>GSHMEPPPKLVLDLERLAHVPQEKAGPLQRYAATIQSQRGDYNGKVLSIRQDDLRTLAVIYDQSPSVLTEQLISWGVLDADARRAVAHEEN[2x]

Here, we report that c-di-GMP can assemble into a tetramer that mediates the effective dimerization of a transcription factor, BldD, which controls the progression of multicellular differentiation in sporulating actinomycete bacteria. BldD is an 18 kDa DNA-binding protein consisting of two distinct domains connected by a flexible linker. BldD sits at the top of the regulatory cascade controlling development, serving to repress expression of sporulation genes during vegetative growth (den Hengst et al., 2010). Specifically, structural and biochemical analyses show that the second messenger c-di-GMP activates BldD DNA binding by driving a unique form of dimerization that is mediated by a tetrameric form of c-di-GMP.

To elucidate the molecular basis for c-di-GMP recognition and binding by the BldD CTD and to gain insight into how this interaction may elicit developmental signaling, we determined structures of the S. venezuelae BldD CTD (residues 80–166) and S. coelicolor BldD CTD (residues 80–167) in complex with c-di-GMP. Three S. venezuelae BldD C-domain-(c-di-GMP) structures and one S. coelicolor BldD C-domain-(c-di-GMP) structure were determined to resolutions of 1.95 Å, 2.33 Å, 1.75 Å, and 2.25 Å, respectively (see Extended Experimental Procedures and Tables S1 and S2). The BldD CTD structures are composed of two (β-α-α) repeats followed by a short C-terminal helix and are similar to the apo form studied by NMR (Kim et al., 2014). The BldD CTD uses a previously unseen mode of c-di-GMP binding in which two noninteracting CTDs are glued together by a c-di-GMP tetramer composed of two interlocked c-di-GMP dimers. The guanine bases wedged between the two motif 2 regions are specified by contacts from residues Arg125 and Asp128. Residue Asp128 makes two hydrogen bonds to the N1 and the exocyclic N2 atoms of the guanine bases on each end (top and bottom layers) of the intercalated dimer, while Arg125 flanks the guanines in the center (middle layers) of the dimer and makes hydrogen bonds to the guanine O6 and N7 atoms. In addition to contacts from Arg114, Asp116 of motif 1 hydrogen bonds to the guanine N1 and N2 atoms in a manner analogous to the contacts from Asp128 of motif 2. While the arginine and aspartic acid residues in BldD motifs 1 and 2 dictate the c-di-GMP-binding arrangement and read the guanine bases, contacts to the c-di-GMP phosphate groups are provided by Lys84 from β1 and Arg130 from α3. Rather, the c-di-GMP molecules are closely spaced and optimally positioned for interbase pairing, leading to the formation of a multistranded, base-stacked structure with top, middle, and bottom layers. There are 12 hydrogen bonds between the two intercalated dimers within the c-di-GMP tetramer, including contacts between the N3 atoms and exocyclic NH2 amides of an adjacent base.> LLIPKVWVPPEDPLASPSRLAKFLRENGYKVLQPRSLPENEEYETDQILPDLAWMRQIEGAVLKPTLSLPIGDQEYFPKYYPTHRPSKEKPNAYPPDIALLKQMIYLFLQVPEANEGLKDEVTLLTQNIRDKAYGSGTYMGQATRLVAMKEVATGRNPNKDPLKLGYTFESIAQLLDITLPVGPPGEDDKPWVPLTRVPSRMLVLTGDVDGDFEVEDYLPKINLKSSSGLPYVGRTKGETIGEMIAISNQFLRELSTLLKQGAGTKGSNKKKLLSMLSDYWYLSCGLLFPKAERYDKSTWLTKTRNIWSAPSPTHLMISMITWPVMSNSPNNVLNIEGCPSLYKFN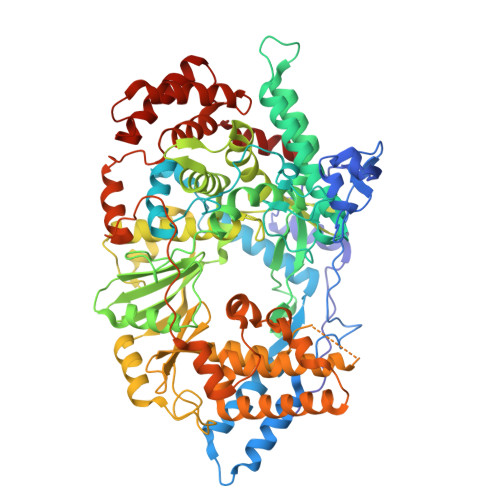PFRGGLNRIVEWILAPEEPKALVYADNIYIVHSNTWYSIDLEKGEANCTRQHMQAAMYYILTRGWSDNGDPMFNQTWATFAMNIAPALVVDSSCLIMNLQIKTYGQGSGNAATFINNHLLSTLVLDQWNLMRQPRPDSEEFKSIEDKLGINFKIERSIDDIRGKLRQLVLLAQPGYLSGGVEPEQSSPTVELDLLGWSATYSKDLGIYVPVLDKERLFCSAAYPKGVENKSLKSKVGIEQAYKVVRYEALRLVGGWNYPLLNKACKNNAGAARRHLEAKGFPLDEFLAEWSELSEFGEAFEGFNIKLTVTSESLAELNKPVPPKPPNVNRPVNTGGLKAVSNALKTGRYRNEAGLSGLVLLATARSRLQDAVKAKAEAEKLHKSKPDDPDADWFERSETLSDLLEKADIASKVAHSALVETSDALEAV>MSQLQHNIGLSIFEPVAKHRANRIICTIGPSTQSVEALKGLMKSGMSVARMNFSHGSYEYHQTTINNVRAAAAELGLHIGIALDTKGPEIRTGLFKDGEATYAPGDTVLVTTDPAFEKIGTKEKFYVDYPQLPNVVRPGGLIYVDDGVLTLRVLSKEDDCTLKCHVNNHHRLTDRKGINLPGCEVDLPAVSEKDRKDLQFGVEQ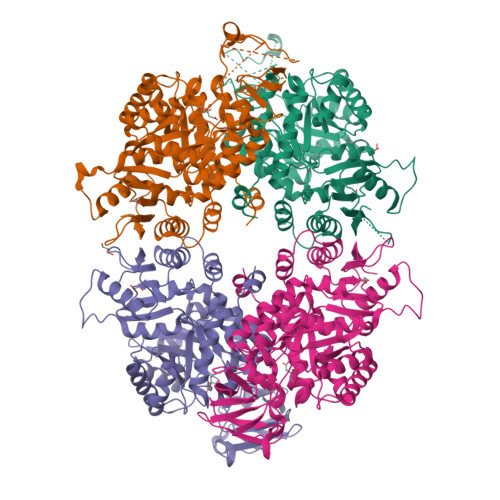GVDMIFASFIRTADQVREVRAALGEKGKDTLIISKIENHQGVQNIDAIIEASDGIMVARGDLGVEIPAEKVVVAQMCIISKCNVAGKPVICATQMLESMTTNPRPTRAEVTDVANAVFNGADCVMLSGETAKGKYPNEVVQYMVRICIEAQSATHDSVMFNSIKNLQKIPMSPEEAVCSSAVSSAFEVQAKAILVLSNTGRSARLISKYRPNCPIICATTRLLTCRQLNVTRSVESVYYDVDAHGEDNDREKRVQLGVDWAKTKGYVSAGDVMVIVHADHSVKGYPNQTRLVRVRENLYFQSGGHHHHHH[8x]> MSRLDKSKVINSALELLNEVGIEGLTTRKLAQKLGVEQPTLYWHVKNKRALLDALAVEILARHHDYSLPAAGESWQSFLRNNAMSFRRALL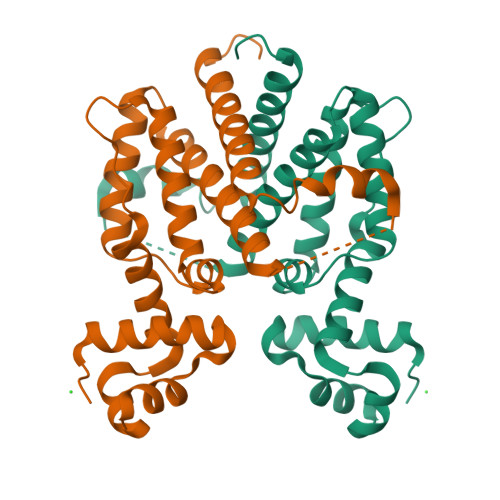RYRDGAKVHLGTRPDEKQYDTVETQLRFMTENGFSLRDGLYAISWVSHFTLGAVLEQQEHTAALTDRPAAPDENLPPLLREALQIMDSDDGEQAFLHGLESLIRGIEVQLTALLQIV5-[(5-fluoro-3-methyl-1H-indazol-4-yl)oxy]benzene-1,3-dicarbonitrile 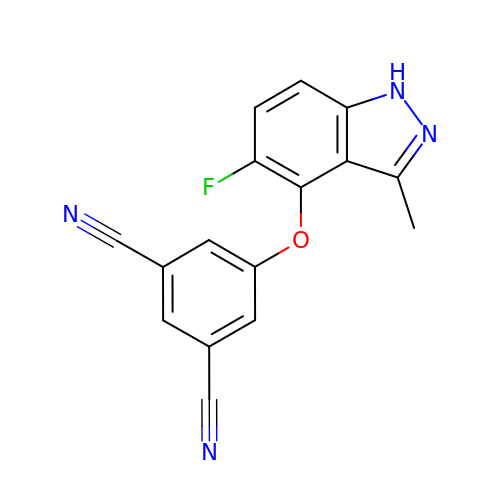| C16 H9 F N4 O | JYAHFMKZJRVTDT-UHFFFAOYSA-N>[2x]MIIGYARVSSLDQ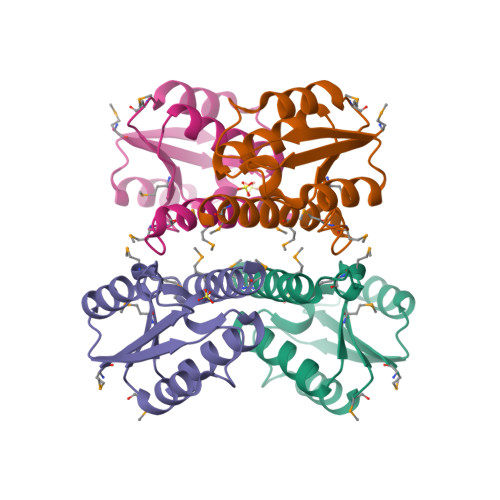NLERQLENLKTFGAEKIFTEKQSGKSIENRPILQKALNFVEMGDRFIVESIDRLGRNYNEVIHIVNYLKDKEVQLMITSLPMMNEVTGNPLLDKFMKDLIIRILAMVSEQERNES> MIEVSEVIAKVRERLNDNEVGNYEILDSVLVENINQALLKICLEFRLKKAITRSLITEEERFLTLNNLLGIESVKLDKKEIESRNTIEKDTGELELLILSDRISVTPFKIGELEVVYYTYEEIRNILETIKLPKICLD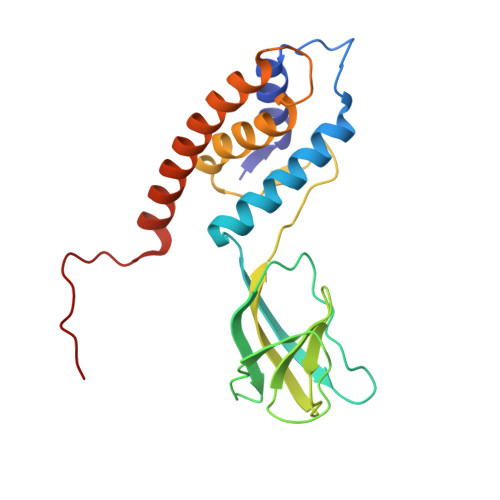VLVYSVLCNLLEIPNNETNFSVLANYKQLLKLAKDNLTNYLSLMYSKNIHFSKVVRV>CGIWALFGSDDCLSVQCLSAMKIAHRGPDAFRFENVNGYTNCCFGFHRLAVVDPLFGMQPIRVKKYPYLWLCYNGEIYNHKKMQQHFEFEYQTKVDGEIILHLYDKGGIEQTICMLDGVFAFVLLDTANKKVFLGRDTYGVIPLFKAMTEDGFLAVCSEAKGLVTLKHSATPFLKVEPFLPGHYEVLDLKPNGKVASVEMVKYHHCRDVPLHALYDNVEKLFPGFEIETVKNNLRILFNNAVKKRLMTDRRIGCLLSGGLDSSLVAATLLKQLKEAQVQYPLQTFAIGMEDSPDLLAARKVADHIGSEHYEVLFNSEEGIQALDEVIFSLETYDITTVRASVGMYLISKYIRKNTDSVVIFSGEGSDELTQGYIYFHKAPSPEKAEEESERLLRELYLFDVLRADRTTAAHGLELRVPFLDHRFSSYYLSLPPEMRIPKNGIEKHLLRETFEDSNLIPKEILWRPKEAFSDGITSVKNSWFKILQEYVEHQVDDAMMANAAQKFPFNTPKTKEGYYYRQVF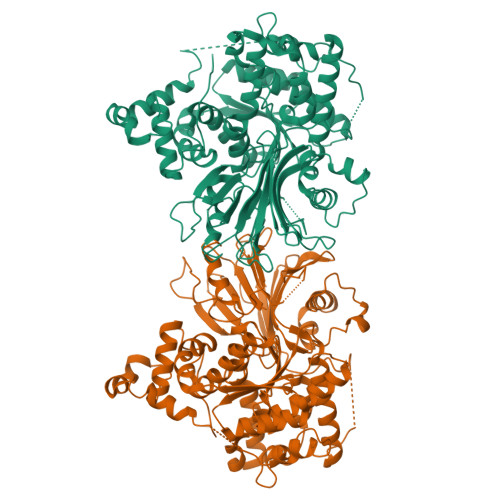ERHYPGRADWLSHYWMPKWINATDPSARTLTHYKSAVKAAGENLYFQSHHHHHHHHHH[2x]> SYS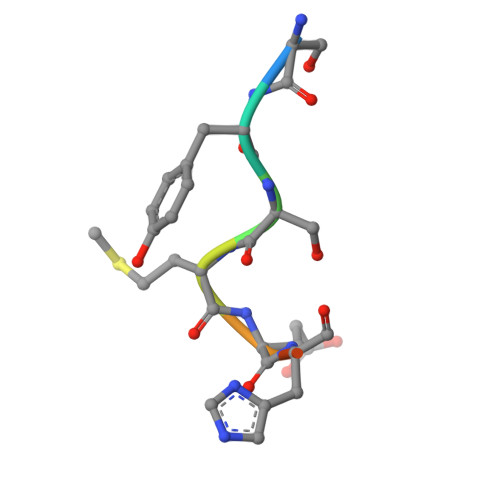MEHFR3-fluoro-N-[(oxan-4-yl)methyl]pyridin-2-amine | C11 H15 F N2 O | 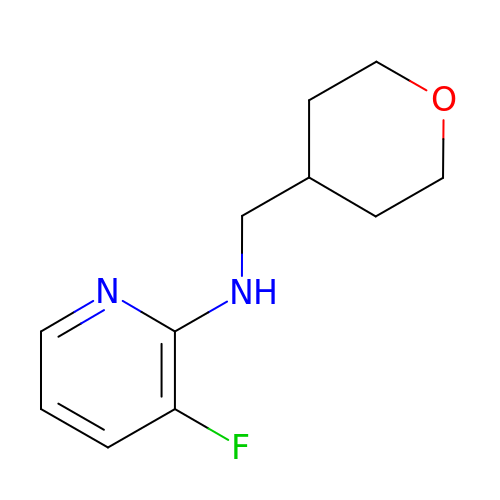RDLLIXJKRKAZRZ-UHFFFAOYSA-N> GSHMSNTQTVLPFTGLNTPNGVAVDSAGTVYVTDHGNNRVVKLAAGSNTQTVLPFTGLNTPNGVAVDSAGTVY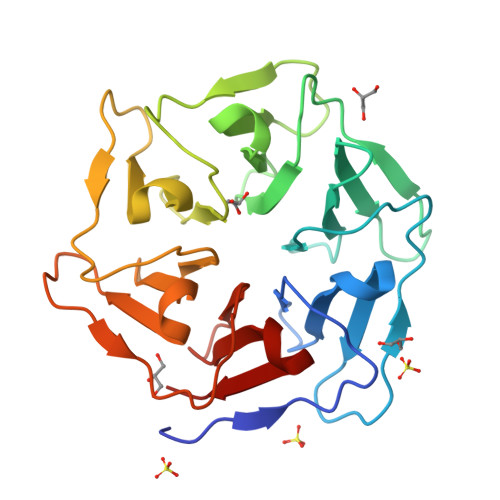VTDHGNNRVVKLAAGSNTQTVLPFTGLNTPNGVAVDSAGTVYVTDHGNNRVVKLAAGSNTQTVLPFTGLNTPNGVAVDSAGTVYVTDHGNNRVVKLAAGSNTQTVLPFTGLNTPNGVAVDSAGTVYVTDHGNNRVVKLAAGSNTQTVLPFTGLNTPNGVAVDSAGTVYVTDHGNNRVVKLAAG> MDKKTIYFISTGNSARSQMAEGWGKEILGEGWNVYSAGIETHGVNPKAIEAMKEVDIDISNHTSDLIDNDILKQSDLVVTLCSDADNNCPILPPNVKKEHWGFDDPAGKE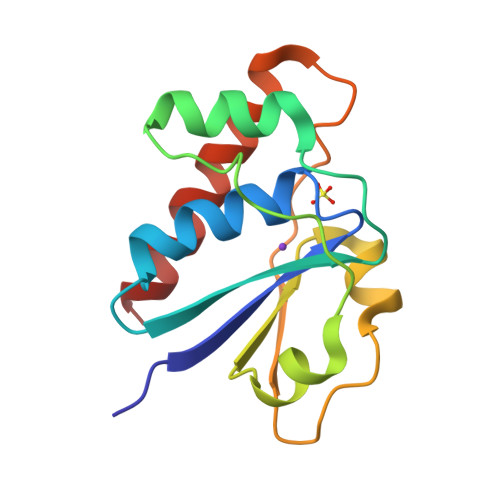WSEFQRVRDEIKLAIEKFKLR> SNANNVENEKSWEKYFAEYKVEGCFMLFNNSQGTFKVYNLERSQQRFLPASTFKIFNSLVGLETGVIKDTSFVIPWDGVTRDMPEWNHDLSMQQAFRVSAVPYFQEVARRITKPVMQHWLDTVKFGNMKISKIDTFWLDNSLQISPDEELGFVKKLYFDQLPFHKVTMQNVRQVMLMEKKPEYELSYKTGMGFSGPKTIGWITGWIEENGHPSFFVLNIETENKSLDMRTVRMNI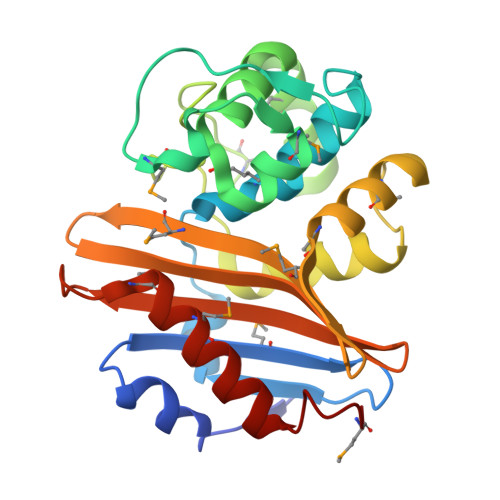LRNLLTDAGYFKGMK> MEASRRDFISIGIGALGAVGGLGALYALVRVMLEPSEIAALGAKTEIDVSKIQPMQVRVTSWKGKTLFAIRLPKDFKPEGYTLKKGALNSKGTTNYEILKGHDVFALVGVCTHLGCIPLWKPQGEGGINKPVFHCPCHGGLYTPYGDVIGGPPPRPLFIPPQKLEGNKLIVGVEGFV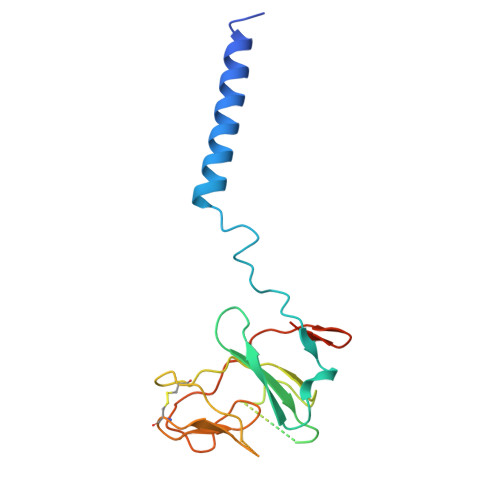KELI> GNASSIVQTINVTGDGN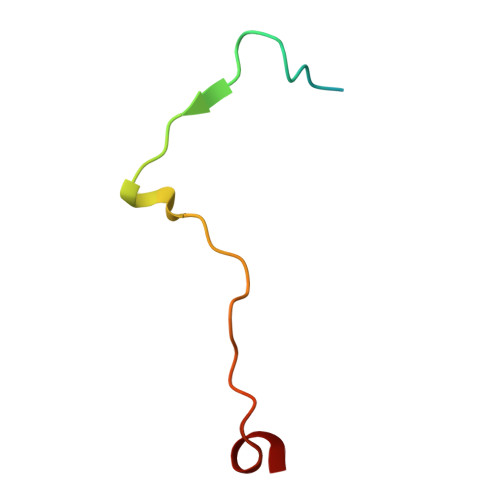VFKPSAETSSTAVPSLSLSPGMLN>GMASLKAKVLETFLAKSRPELLEYYIKVILDYNTAHNKVALSECYTVASVAEMPQNYRPHPQRFTYCSQVLGLHCYKKGIHYWEVELQKNNFCGVGICYGSMNRQGPESRLGRNSASWCVEWFNTKISAWHNNVEKTLPSTKATRVGVLLNCDHGFVIFFAVADKVHLMYKFRVDFTEALYPAFWVFSAGATLSICSPK[3x]

Tripartite motif (TRIM) family proteins are RING-type E3 ligases that play key regulatory roles in innate immune signalling pathways that lead to the induction of a type I interferon (IFN) response and production of inflammatory cytokines through activation of the IRF3 and NF-κB transcription factors. Activation of RIG-I initiates a signalling cascade that depends on the E3 ligase activity of TRIM25 and induces the production of IFNs and inflammatory cytokines. An example is non-structural protein 1 (NS1) of influenza A viruses (IAV), a multifunctional virulence factor that binds many host proteins during infection, including TRIM2527–29. To understand NS1-mediated inhibition of TRIM25 activity on a molecular level we have determined crystal structures of the CC domain of TRIM25 in complex with NS1-FL and the isolated ED, and of a TRIM25 CC-PRYSPRY fragment, which includes the RIG-I-recognition domain of TRIM25.

In parallel we performed NMR titrations between the separate CC and PRYSPRY domains. These experiments show that the interaction between the two domains is weak in solution but involves the interface observed in the crystal structure as mutation of Y463S and Y476S weakened the interaction even further. The functional importance of this interface for the correct positioning of the PRYSPRY to enable substrate ubiquitination is highlighted by the almost complete loss of RIG-I-2CARD ubiquitination upon mutation of these residues although the overall fold of the PRYSPRY domain remains intact. Taken together, these experiments suggest that in the absence of other components of the system, the PRYSPRY domain is in a dynamic equilibrium between a bound state and a constrained diffusing state tethered to the CC by the flexible linker, in agreement with recent results, but that the bound state is important to enable substrate ubiquitination.[(1R,5S)-8-methyl-8-azabicyclo[3.2.1]octan-3-yl] (2S)-3-oxidanyl-2-phenyl-propanoate | C17 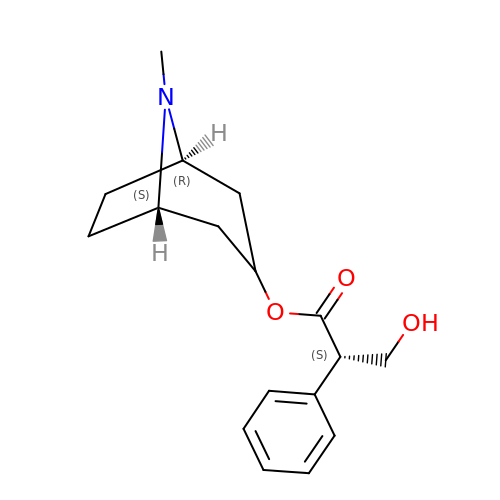H23 N O3 | RKUNBYITZUJHSG-QKPAOTATSA-N>[2x]TVNQAKIFAQTTKMLEFAKQLLETDDFSTLREAYYVSKNWGEARFDDQQASNNVIEDLEAALGVLREHLGFIPEEDGSSVVGPLKIIEETPEGELVVDCTK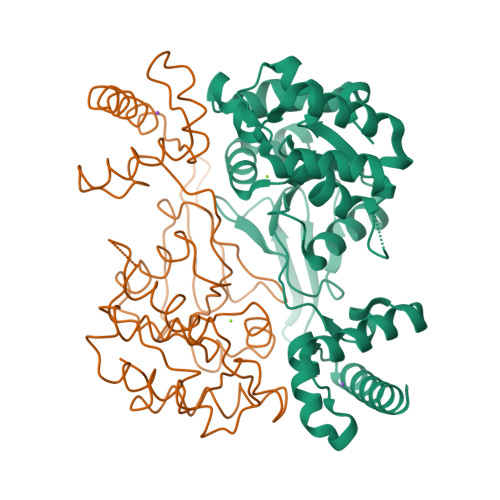LGTGAYNIPNDVTKLNLETDADFILAIETSGMFARLNAERFWDKHNCILVSLKGVPARATRRFIKRLHEEHDLPVLVFTDGDPYGYLNIYRTLKVGSGKAIHLADKLSIPAARLIGVTPQDIIDYDLPTHPLKEQDIKRIKDGLKNDDFVRSFPEWQKALKQMLDMGVRAEQQSLAKYGLKYVVNTYLPEKIKDESTWLP>DGGFCEVCKKLVGYLDRNLEKNSTKQEILAALEKGCSFLPDPYQKQCDQFVAEYEPVLIEILVEVMDPSFV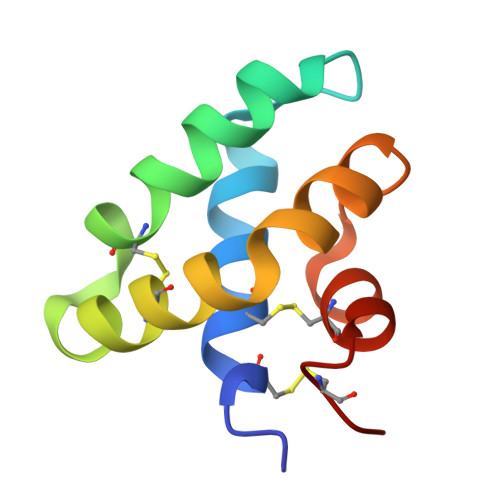CLKIGACPS[4x]>[4x]DMPVEKIQEAEMAVEPKDGN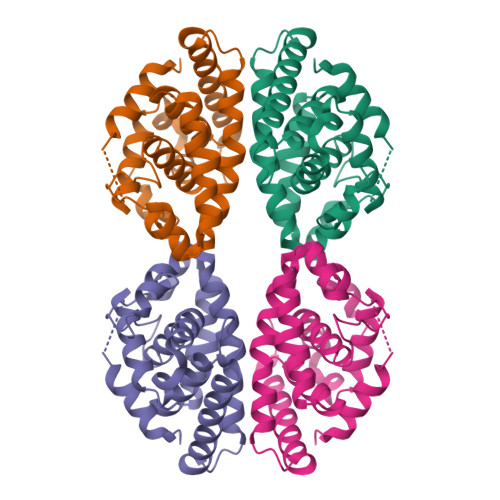MVEQPNDPVTNICQAADKQLVTLVEWAKRIPHFSDLPIDDQVILLRAGWNELLIAAFSHRSIDVKDGILLASGLHVHRSSAHQAGVGTIFDRVLTELVAKMRDMKMDKTELGCLRAIVLFNPDAKGLTDPSLVESLREKVYASLEEYCKQQYPEQPGRFAKLLLRLPALRSIGLKCLEHLFFFKLIGDTPIDTFLMEML6-bromanylspiro[3~{H}-chromene-2,4'-piperidine]-4-one | C13 H14 Br N O2 | 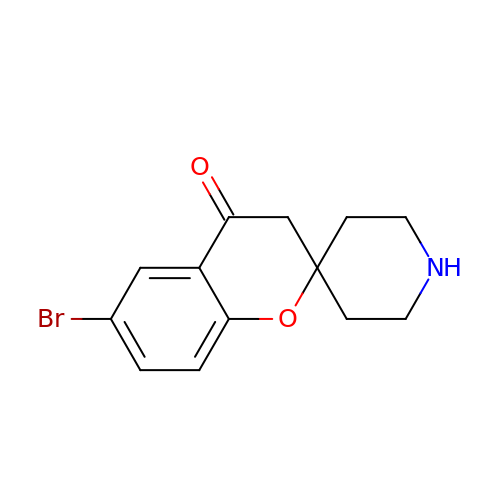HTOKNOIQHUEHNB-UHFFFAOYSA-N> 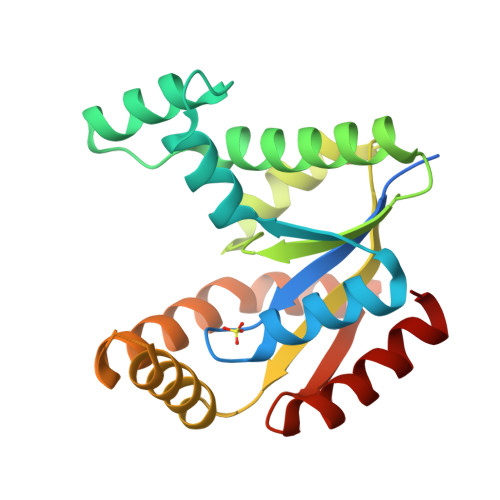MGSSHHHHHHENLYFQGGMKPLVVFVLGGPGAGKGTQCARIVEKYGYTHLSAGELLRDERKNPDSQYGELIEKYIKEGKIVPVEITISLLKREMDQTMAANAQKNKFLIDGFPRNQDNLQGWNKTMDGKADVSFVLFFDCNNEICIERCLERGKSSGRSDDNRESLEKRIQTYLQSTKPIIDLYEEMGKVKKIDASKSVDEVFDEVVQIFDKEG> FLPPVGVENREPADATIREKRAKIKEMMTHAWNNYKRYAWGLNELKPISKEGHSSSLFGNIKGATIVDALDTLFIMGMKTEFQEAKSWIKKYLDFNVNAEVSV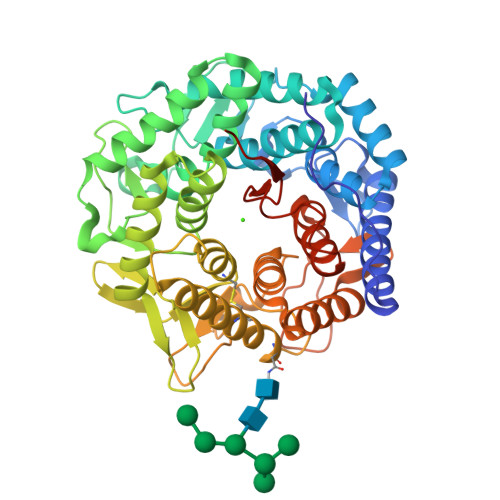FEVNIRFVGGLLSAYYLSGEEIFRKKAVELGVKLLPAFHTPSGIPWALLNMKSGIGRNWPWASGGSSILAEFGTLHLEFMHLSHLSGDPVFAEKVMKIRTVLNKLDKPEGLYPNYLNPSSGQWGQHHVSVGGLGDSFYEYLLKAWLMSDKTDLEAKKMYFDAVQAIETHLIRKSSGGLTYIAEWKGGLLEHKMGHLTCFAGGMFALGADGAPEARAQHYLELGAEIARTCHESYNRTYVKLGPEAFRFDGGVEAIATRQNEKYYILRPEVIETYMYMWRLTHDPKYRTWAWEAVEALESHCRVNGGYSGLRDVYIARESYDDVQQSFFLAETLKYLYLIFSDDDLLPLEHWIFNTEAHPFPILREQKKEIDGKEK> SPSAQELKEQGNRLFVGRKYPEAAACYGRAITRNPLVAV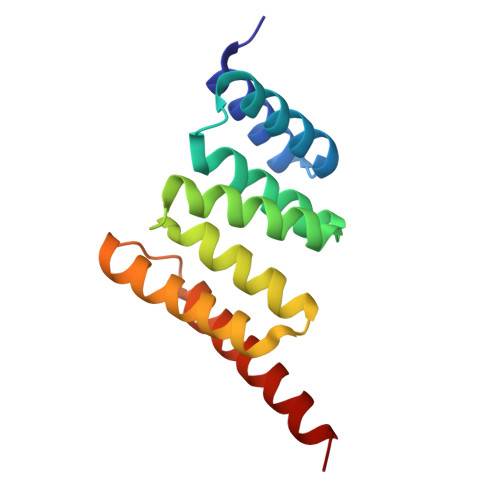YYTNRALCYLKMQQHEQALADCRRALELDGQSVKAHFFLGQCQLEMESYDEAIANLQRAYSLAKEQRLNFGDDIPSALRIAKKKRWNSIEERR>MRPLKVALVNIPLRVPGSDAWISVPPQGYGGIQWVVANLMDGLLELGHEVFLLGAPGSPAGRPGLTVVPAGEPEEIERWLRTADVDVVHDHSGGVIGPAGLPPGTAFISSHHFTTRPVNPVGCTYSSRAQRAHCGGGDDAPVIPIPVDPARYRSAADQVAKEDFLLFMGRVSPHKGALEAAAFAHACGRRLVLAGPAWEPEYFDEITRRYGSTVEPIGEVGGERRLDLLASAHAVLAMSQAVTGPWGGIWCEPGATVVSEAAVSGTPVVGTGNGCLAEIVPSVGEVVGYGTDFAPDEA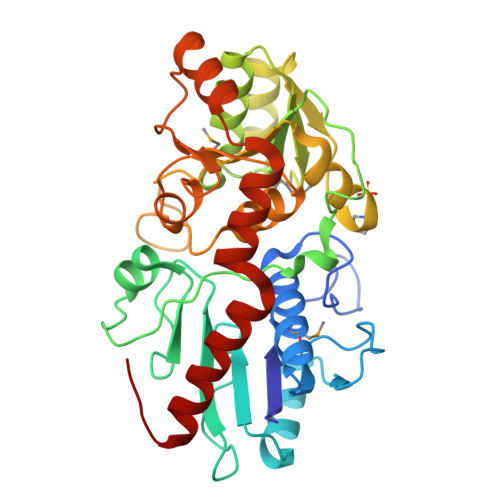RRTLAGLPASDEVRRAAVRLWGHVTIAERYVEQYRRLLAGATWK[2x]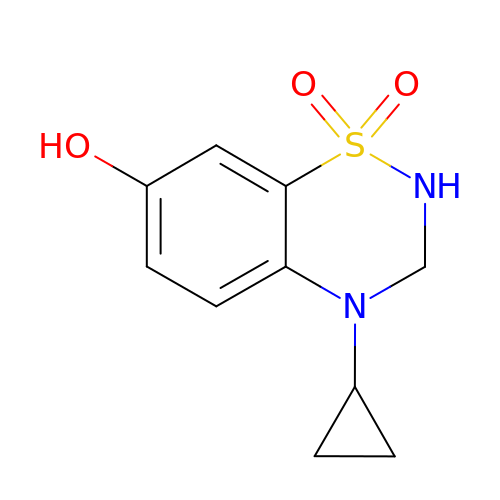4-Cyclopropyl-3,4-dihydro-7-hydroxy-2H-1,2,4-benzothiadiazine 1,1-dioxide | C10 H12 N2 O3 S | OMEAYSCNDLQLNC-UHFFFAOYSA-N> QDVRVRVLPEVRGRLGGTVELPCHLLPPTTERVSQVTWQRLDGTVVAAFHPSFGVDFPNSQFSKDRLSFVRARPETNADLRDATLAFRGLRVEDEGNYTCEFATDPNGTRRGVTWLRVIAQPENHAEAQEVTIGPQSVAVARC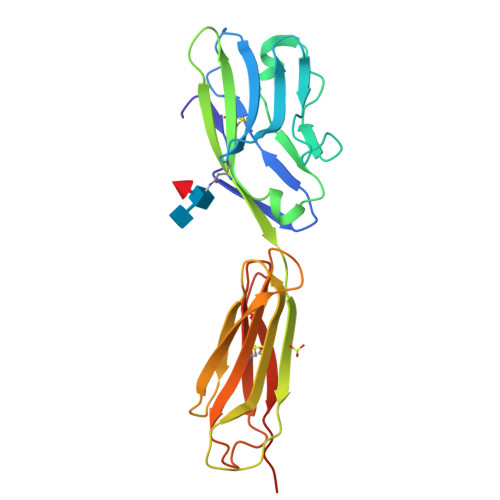VSTGGRPPARITWISSLGGEAKDTQEPGIQAGTVTIISRYSLVPVGRADGVKVTCRVEHESFEEPILLPVTLSVRYHHHHHH>[2x]MKGQETRGFQSEVKQLLHLMIHSLYSNKEIFLRELISNASDAADKLRFRALSNPDLYEGDGELRVRVSFDKDKRTLTISDNGVGMTRDEVIDHLGTIAKSGTKSFLESLGSDQAKDSQLIGQFGVGFYSAFIVADKVTVRTRAAGEKPENGVFWESAGEGEYTVADITKEDRGTEITLHLREGEDEFLDDWRVRSIISKYSDHIALPVEIEKREEKDGETVISWEKINKAQALWTRNKSEITDEEYKEFYKHIAHDFNDPLTWSHNRVEGKQEYTSLLYIPSQAPWDMWNRDHKHGLKLYVQRVFIMDDAEQFMPNYLRFVRGLIDSSDLPLNVSREILQDSTVTRNLRNALTKRVLQMLEKLAKDDAEKYQTFWQQFGLVLKEGPAEDFANQEAIAKLLRFASTHTDSSAQTVSLEDYVSRMKEGQEKIYYITADSYAAAKSSPHLELLRKKGIEVLLLSDRIDEWMMNYL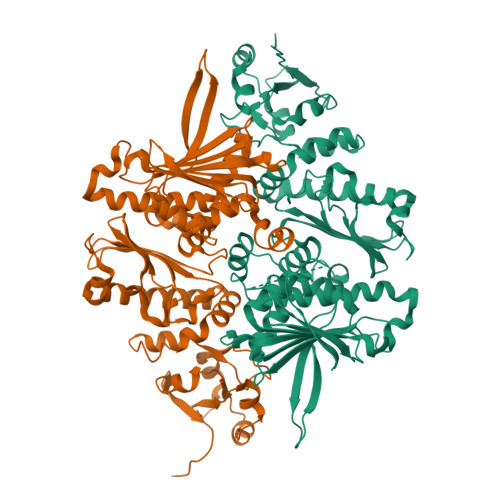TEFDGKPFQSVSKVDESLEKLADEVDESAKEAEKALTPFIDRVKALLGERVKDVRLTHRLTDTPAIVSTDADEMSTQMAKLFAAAGQ> MISKRLELVASFVSQGAILLDVGSDHAYLPIELVERGQIKSAIAGEVVEG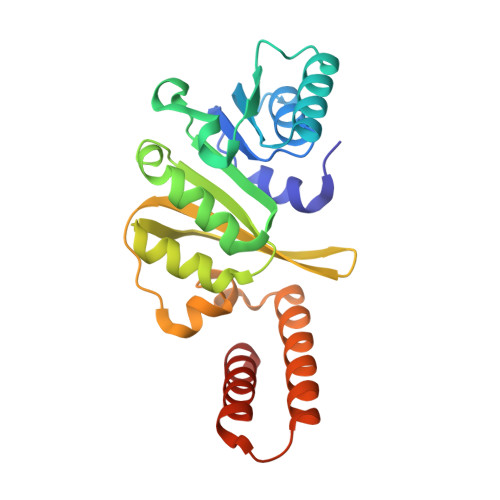PYQSAVKNVEAHGLKEKIQVRLANGLAAFEETDQVSVITIAGMGGRLIARILEEGLGKLANVERLILQPNNREDDLRIWLQDHGFQIVAESILEEAGKFYEILVVEAGQMKLSASDVRFGPFLSKEVSPVFVQKWQKEAEKLEFALGQIPEKNLEERQVLVDKIQAIKEVLHVSK3-{4-amino-1-[(3S)-1-propanoylpiperidin-3-yl]-1H-pyrazolo[3,4-d]pyrimidin-3-yl}-N-[4-(propan-2-yl)phenyl]benzamide | C29 H33 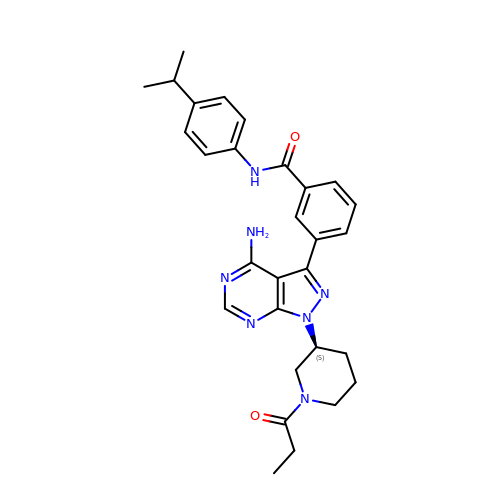N7 O2 | OQUNLLPGZMGVNR-QHCPKHFHSA-N> SVEDSLQNPEVAVAACNAFLEANYPXXXXXXXXXXXXXXXXXXXXXXXXXXXXXXXXXXXXXXXXXXXXXXXXXXSAVPSPFANTLANVLAAATKRNCNVTQMRELPTLDSAVLNVECFKKFACNGEYWQEFKDNPIRITTENITTYVTRLKGPKAAALFAKTHNLVPLQEVPMDRFVVDMKRDVKVTPGTKHTEERPKVQVIQAAEPLATAYLCGIHRELVRRLKAVLAPNIHTLFDMSAEDFDAIIAAHFQPGDAVLETDIASFDKSQDDSLALTALMLLEDLGVDQELLDLIEAAFGEITSVHLPTGTRFKFGAMMKSGMFLTLFVNTLLNIVIACRVL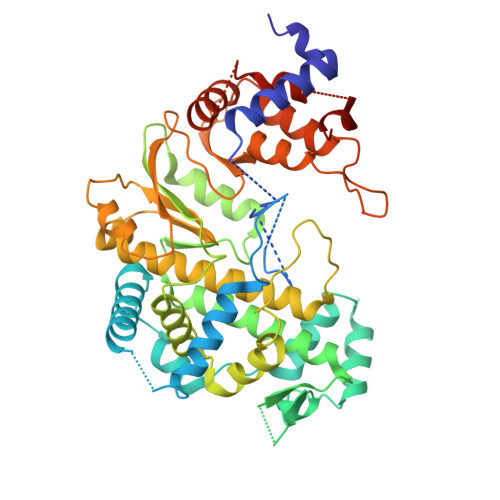REKLTNSVCAAFIGDDNIVHGVRSDPLMAERCASWVNMEVKIIDATMCEKPPYFCGGFILYDKVTGSACRVADPLKRLFKLGKPLPAGDTQDEDRRRALKDETDRWARVGLKSELEIALSSRYEVNGTGNIVRAMATLAKSLKNFKKLRGPIVHLYGGPK>[2x]MDYKDDDDKLAAANSSIDLISTSLYKKAGLTMVTGGGAAPPGTVTEPLPSVIVLSAGRKMAAAAAAASGPGCSSAAGAGAAGVSEWLVLRDGCMHCDADGLHSLSYHPALNAILAVTSRGTIKVIDGTSGATLQASALSAKPGGQVKCQYISAVDKVIFVDDYAVGCRKDLNGILLLDTALQTPVSKQDDVVQLELPVTEAQQLLSACLEKVDISSTEGYDLFITQLKDGLKNTSHETAANHKVAKWATVTFHLPHHVLKSIASAIVNELKKINQNVAALPVASSVMDRLSYLLPSARPELGVGPGRSVDRSLMYSEANRRETFTSWPHVGYRWAQPDPMAQAGFYHQPASSGDDRAMCFTCSVCLVCWEPTDEPWSEHERHSPNCPFVKGEHTQNVPLSVTLATSPAQFPCTDGTDRISCFGSGSCPHFLAAATKRGKICIWDVSKLMKVHLKFEINAYDPAIVQQLILSGDPSSGVDSRRPTLAWLEDSSSCSDIPKLEGDSDDLLEDSDSEEHSRSDSVTGHTSQKEAMEVSLDITALSILQQPEKLQWEIVANVLEDTVKDLEELGANPCLTNSKSEKTKEKHQEQHNIPFPCLLAGGLLTYKSPATSPISSNSHRSLDGLSRTQGESISEQGSTDNESCTNSELNSPLVRRTLPVLLLYSIKESDEKAGKIFSQMNNIMSKSLHDDGFTVPQIIEMELDSQEQLLLQDPPVTYIQQFADAAANLTSPDSEKWNSVFPKPGTLVQCLRLPKFAEEENLCIDSITPCADGIHLLVGLRTCPVESLSAINQVEALNNLNKLNSALCNRRKGELESNLAVVNGANISVIQHESPADVQTPLIIQPEQRNVSGGYLVLYKMNYATRIVTLEEEPIKIQHIKDPQDTITSLILLPPDILDNREDDCEEPIEDMQLTSKNGFEREKTSDISTLGHLVITTQGGYVKILDLSNFEILAKVEPPKKEGTEEQDTFVSVIYCSGTDRLCACTKGGELHFLQIGGTCDDIDEADILVDGSLSKGIEPSSEGSKPLSNPSSPGISGVDLLVDQPFTLEILTSLVELTRFETLTPRFSATVPPCWVEVQQEQQQRRHPQHLHQQHHGDAAQHTRTWKLQTDSNSWDEHVFELVLPKACMVGHVDFKFVLNSNITNIPQIQVTLLKNKAPGLGKVNALNIEVEQNGKPSLVDLNEEMQHMDVEESQCLRLCPFLEDHKEDILCGPVWLASGLDLSGHAGMLTLTSPKLVKGMAGGKYRSFLIHVKAVNERGTEEICNGGMRPVVRLPSLKHQSNKGYSLASLLAKVAAGKEKSSNVKNENTSGTRKSENLRGCDLLQEVSVTIRRFKKTSISKERVQRCAMLQFSEFHEKLVNTLCRKTDDGQITEHAQSLVLDTLCWLAGVHSNGPGSSKEGNENLLSKTRKFLSDIVRVCFFEAGRSIAHKCARFLALCISNGKCDPCQPAFGPVLLKALLDNMSFLPAATTGGSVYWYFVLLNYVKDEDLAGCSTACASLLTAVSRQLQDRLTPMEALLQTRYGLYSSPFDPVLFDLEMSGSSCKNVYNSSIGVQSDEIDLSDVLSGNGKVSSCTAAEGSFTSLTGLLEVEPLHFTCVSTSDGTRIERDDAMSSFGVTPAVGGLSSGTVGEASTALSSAAQVALQSLSHAMASAEQQLQVLQEKQQQLLKLQQQKAKLEAKLHQTTAAAAAAASAVGPVHNSVPSNPVAAPGFFIHPSDVIPPTPKTTPLFMTPPLTPPNEAVSVVINAELAQLFPGSVIDPPAVNLAAHNKNSNKSRMNPLGSGLALAISHASHFLQPPPHQSIIIERMHSGARRFVTLDFGRPILLTDVLIPTCGDLASLSIDIWTLGEEVDGRRLVVATDISTHSLILHDLIPPPVCRFMKITVIGRYGSTNARAKIPLGFYYGHTYILPWESELKLMHDPLKGEGESANQPEIDQHLAMMVALQEDIQCRYNLACHRLETLLQSIDLPPLNSANNAQYFLRKPDKAVEEDSRVFSAYQDCIQLQLQLNLAHNAVQRLKVALGASRKMLSETSNPEDLIQTSSTEQLRTIIRYLLDTLLSLLHASNGHSVPAVLQSTFHAQACEELFKHLCISGTPKIRLHTGLLLVQLCGGERWWGQFLSNVLQELYNSEQLLIFPQDRVFMLLSCIGQRSLSNSGVLESLLNLLDNLLSPLQPQLPMHRRTEGVLDIPMISWVVMLVSRLLDYVATVEDEAAAAKKPLNGNQWSFINNNLHTQSLNRSSKGSSSLDRLYSRKIRKQLVHHKQQLNLLKAKQKALVEQMEKEKIQSNKGSSYKLLVEQAKLKQATSKHFKDLIRLRRTAEWSRSNLDTEVTTAKESPEIEPLPFTLAHERCISVVQKLVLFLLSMDFTCHADLLLFVCKVLARIANATRPTIHLCEIVNEPQLERLLLLLVGTDFNRGDISWGGAWAQYSLTCMLQDILAGELLAPVAAEAMEEGTVGDDVGATAGDSDDSLQQSSVQLLETIDEPLTHDITGAPPLSSLEKDKEIDLELLQDLMEVDIDPLDIDLEKDPLAAKVFKPISSTWYDYWGADYGTYNYNPYIGGLGIPVAKPPANTEKNGSQTVSVSVSQALDARLEVGLEQQAELMLKMMSTLEADSILQALTNTSPTLSQSPTGTDDSLLGGLQAANQTSQLIIQLSSVPMLNVCFNKLFSMLQVHHVQLESLLQLWLTLSLNSSSTGNKENGADIFLYNANRIPVISLNQASITSFLTVLAWYPNTLLRTWCLVLHSLTLMTNMQLNSGSSSAIGTQESTAHLLVSDPNLIHVLVKFLSGTSPHGTNQHSPQVGPTATQAMQEFLTRLQVHLSSTCPQIFSEFLLKLIHILSTERGAFQTGQGPLDAQVKLLEFTLEQNFEVVSVSTISAVIESVTFLVHHYITCSDKVMSRSGSDSSVGARACFGGLFANLIRPGDAKAVCGEMTRDQLMFDLLKLVNILVQLPLSGNREYSARVSVTTNTTDSVSDEEKVSGGKDGNGSSTSVQGSPAYVADLVLANQQIMSQILSALGLCNSSAMAMIIGASGLHLTKHENFHGGLDAISVGDGLFTILTTLSKKASTVHMMLQPILTYMACGYMGRQGSLATCQLSEPLLWFILRVLDTSDALKAFHDMGGVQLICNNMVTSTRAIVNTARSMVSTIMKFLDSGPNKAVDSTLKTRILASEPDNAEGIHNFAPLGTITSSSPTAQPAEVLLQATPPHRRARSAAWSYIFLPEEAWCDLTIHLPAAVLLKEIHIQPHLASLATCPSSVSVEVSADGVNMLPLSTPVVTSGLTYIKIQLVKAEVASAVCLRLHRPRDASTLGLSQIKLLGLTAFGTTSSATVNNPFLPSEDQVSKTSIGWLRLLHHCLTHISDLEGMMASAAAPTANLLQTCAALLMSPYCGMHSPNIEVVLVKIGLQSTRIGLKLIDILLRNCAASGSDPTDLNSPLLFGRLNGLSSDSTIDILYQLGTTQDPGTKDRIQALLKWVSDSARVAAMKRSGRMNYMCPNSSTVEYGLLMPSPSHLHCVAAILWHSYELLVEYDLPALLDQELFELLFNWSMSLPCNMVLKKAVDSLLCSMCHVHPNYFSLLMGWMGITPPPVQCHHRLSMTDDSKKQDLSSSLTDDSKNAQAPLALTESHLATLASSSQSPEAIKQLLDSGLPSLLVRSLASFCFSHISSSESIAQSIDISQDKLRRHHVPQQCNKMPITADLVAPILRFLTEVGNSHIMKDWLGGSEVNPLWTALLFLLCHSGSTSGSHNLGAQQTSARSASLSSAATTGLTTQQRTAIENATVAFFLQCISCHPNNQKLMAQVLCELFQTSPQRGNLPTSGNISGFIRRLFLQLMLEDEKVTMFLQSPCPLYKGRINATSHVIQHPMYGAGHKFRTLHLPVSTTL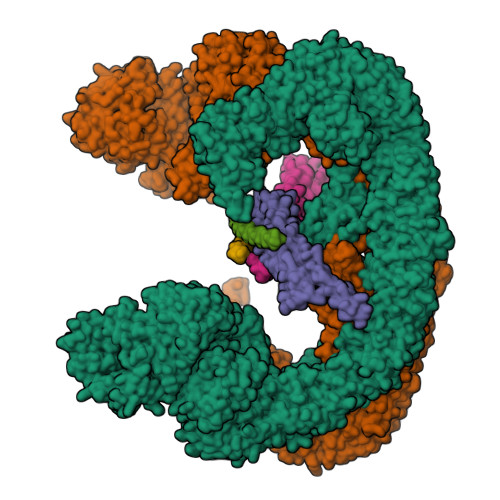SDVLDRVSDTPSITAKLISEQKDDKEKKNHEEKEKVKAENGFQDNYSVVVASGLKSQSKRAVSATPPRPPSRRGRTIPDKIGSTSGAEAANKIITVPVFHLFHKLLAGQPLPAEMTLAQLLTLLYDRKLPQGYRSIDLTVKLGSRVITDPSLSKTDSYKRLHPEKDHGDLLASCPEDEALTPGDECMDGILDESLLETCPIQSPLQVFAGMGGLALIAERLPMLYPEVIQQVSAPVVTSTTQEKPKDSDQFEWVTIEQSGELVYEAPETVAAEPPPIKSAVQTMSPIPAHSLAAFGLFLRLPGYAEVLLKERKHAQCLLRLVLGVTDDGEGSHILQSPSANVLPTLPFHVLRSLFSTTPLTTDDGVLLRRMALEIGALHLILVCLSALSHHSPRVPNSSVNQTEPQVSSSHNPTSTEEQQLYWAKGTGFGTGSTASGWDVEQALTKQRLEEEHVTCLLQVLASYINPVSSAVNGEAQSSHETRGQNSNALPSVLLELLSQSCLIPAMSSYLRNDSVLDMARHVPLYRALLELLRAIASCAAMVPLLLPLSTENGEEEEEQSECQTSVGTLLAKMKTCVDTYTNRLRSKRENVKTGVKPDASDQEPEGLTLLVPDIQKTAEIVYAATTSLRQANQEKKLGEYSKKAAMKPKPLSVLKSLEEKYVAVMKKLQFDTFEMVSEDEDGKLGFKVNYHYMSQVKNANDANSAARARRLAQEAVTLSTSLPLSSSSSVFVRCDEERLDIMKVLITGPADTPYANGCFEFDVYFPQDYPSSPPLVNLETTGGHSVRFNPNLYNDGKVCLSILNTWHGRPEEKWNPQTSSFLQVLVSVQSLILVAEPYFNEPGYERSRGTPSGTQSSREYDGNIRQATVKWAMLEQIRNPSPCFKEVIHKHFYLKRVEIMAQCEEWIADIQQYSSDKRVGRTMSHHAAALKRHTAQLREELLKLPCPEGLDPDTDDAPEVCRATTGAEETLMHDQVKPSSSKELPSDFQL;>MAVPIAQKSEPHSLSSEALMRRAVSLVTDSTSTFLSQTTYALIEAITEYTKAVYTLTSLYRQYTSLLGKMNSEEEDEVWQVIIGARAEMTSKHQEYLKLETTWMTAVGLSEMAAEAAYQTGADQASITARNHIQLVKLQVEEVHQLSRKAETKLAEAQIEELRQKTQEEGEERAESEQEAYLREDHHHHHHHHH[2x]{2-[1-(3-fluoro-4-hydroxyphenyl)-1H-1,2,3-triazol-4-yl]-8-oxo-1,7-naphthyridin-7(8H)-yl}acetic 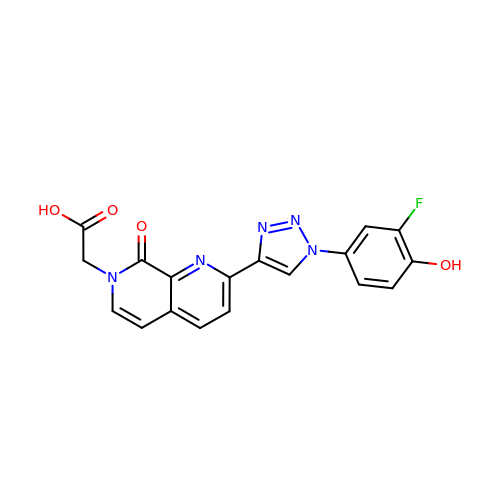acid | C18 H12 F N5 O4 | JIHPTULEFOYNCY-UHFFFAOYSA-N(1s,3s)-N-({4-[5-(2-fluoropropan-2-yl)-1,2,4-oxadiazol-3-yl]bicyclo[2.2.2]octan-1-yl}methyl)-3-hydroxy-N-[4'-(2-hydroxypropan-2-yl)[1,1'-biphenyl]-3-yl]-3-(trifluoromethyl)cyclobutane-1-carboxamide 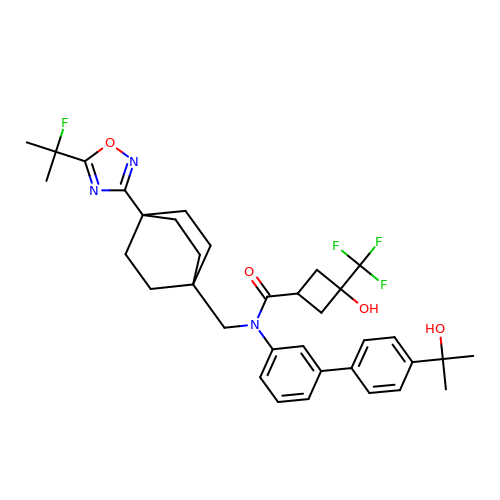| C35 H41 F4 N3 O4 | AEMZJBZKICOPPC-OIFGHDHESA-N>[2x]AMRQCAIYGKGGIGKSTTTQNLVAALAEMGKKVMIVGCDPKADSTRLI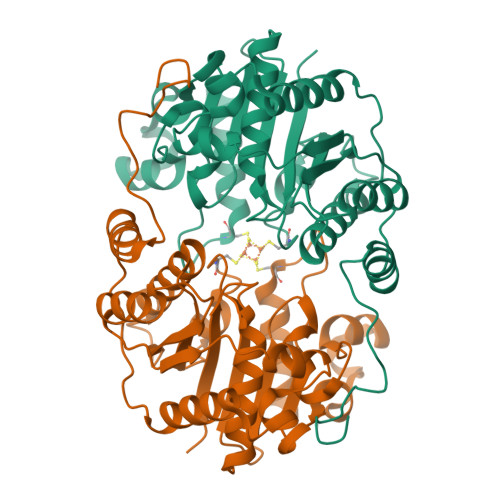LHSKAQNTIMEMAAEAGTVEDLELEDVLKAGYGGVKCVESGGPEPGVGCAGRGVITAINFLEEEGAYEDDLDFVFYDVLGEVVCGGFAMPIRENKAQEIYIVCSGEMMAMYAANNISKGIVKYANSGSVRLGGLICNSRNTDREDELIIALANKLGTQMIHFVPRDNVVQRAEIRRMTVIEYDPKAKQADEYRALARKVVDNKLLVIPNPITMDELEELLMEFGIMEVEDESIVGKTAEEV>[2x]MAHHHHHHMTQLSVNVNKIAVLRNSRGGAEPDVVRAAQACLDAGAHGITVHPRPDRRHITAEDVLALSTLTRARGVEFNIEGNPFAPPREGYPGLLPLCAQTRPAQATLVPDGDGQITSDHGFDFERD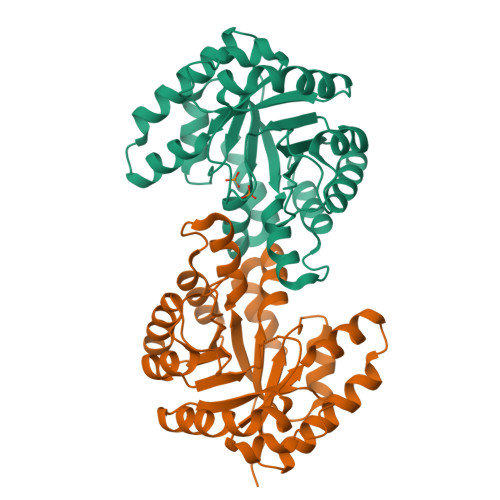AERLRPLVAELKAMGCRVSLFVDAGNPLLEQAAEVGADRVELYTGPYAEAHAAGDAAAMLELFATAARRAQAMGLGVNAGHDLSQDNLRDFLAHVPDVLEVSIGHALIGEALYDGLDATVRGYLALL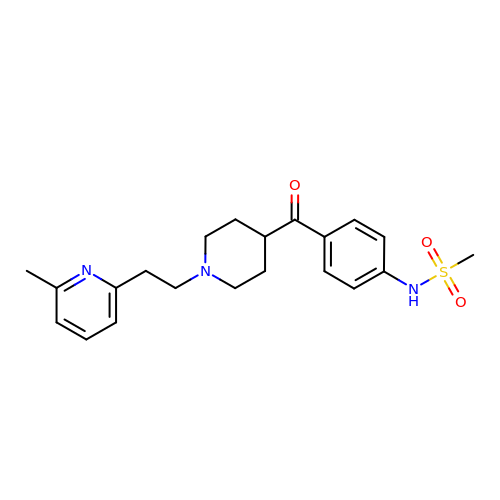~{N}-[4-[1-[2-(6-methylpyridin-2-yl)ethyl]piperidin-4-yl]carbonylphenyl]methanesulfonamide | C21 H27 N3 O3 S | SRUISGSHWFJION-UHFFFAOYSA-N>[2x]MVKLTPELINQSMQYINPVRERELDLRGYKIPQIENLGATLDQFDTIDLSDNDLRKLDNLPHLPRLKTLLLNNNRILRISEGLEEAVPNLGSIILTGNNLQELSDLEPLVGFTKLETISLLINPVSTKPNYREYMAYKFPQLRL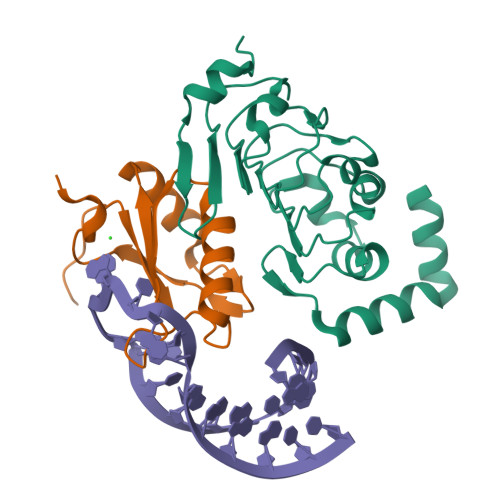LDFRKIKQKDRQAAQEFFRTKQGKDVLKEISR;>[2x]GAMEMLPNQTIYINNLNEKIKKEELKKSLYAIFSQFGQILDIVALKTLKMRGQAFVIFKEIGSASNALRTMQGFPFYDKPMQIAYSKSDSDIVAKIKG>SNAMSKPFMFEKPFGMRDTLPEWYKTKKNICDQMTEEINLWGYDMIETPTLEYYETVGVVSAILDQQLFKLLDQQGNTLVLRPDMTAPIARLVASSLKDRAYPLRLAYQSNVYRAQQNEGGKPAEFEQLGVELIGDGTASADGEVIALMIAALKRAGLSEFKVAIGHVGYVNALLMDVVGNEQRADRLRRFLYEKNYVGYREHVKSLNLSTIDKSRLMNLLSLRGGRAAIEEARGLIQTEKGKTA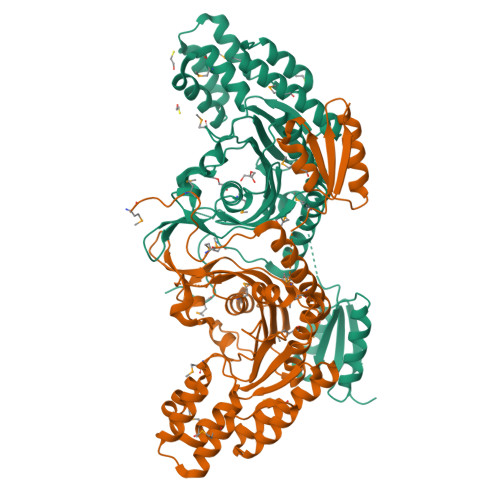LAEMTKLYEVLESYGASEYVKFDLTLVLHMSYYTGVVFEGYGNRLGVPLCSGGRYDELLSKFHRPAQATGFGVRIDLLVEALNGEIISNGHEQTCILFSNERRFEAIELARKKRANGEAVVLQDLAGVTDVDAMSSNYQDVIYCIGTAGRGGEDA[2x]>EEVKAIRIPVVRLKFGEVAEATSVVVLPVCKAEEGEKKILEAPMEIIAGGDFKVVEAEKGWKRWVVLPSWNPVAAIGKGGVAVSFRDDRKVLPWDGKEEPLLVVADRVRNVVEADDGYYLVVAENGLKLE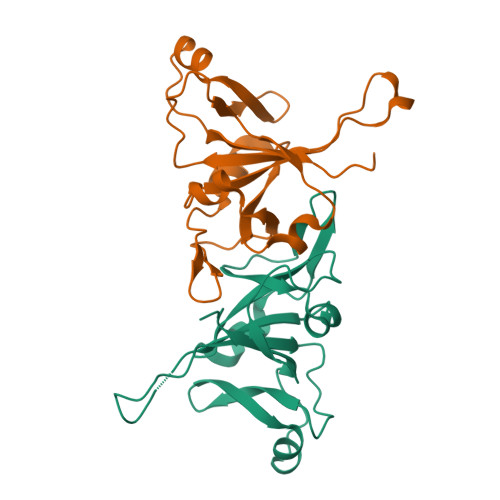KGSDLKAREVKESLGMVVLVVRPPREDDDDWQTSHQNWD[2x]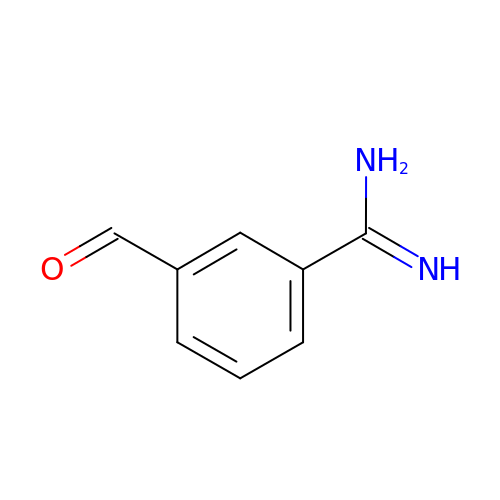3-formylbenzenecarboximidamide | C8 H8 N2 O | GXPBBYFOLVWXRG-UHFFFAOYSA-N(2R)-N-(4-chlorophenyl)-2-[cis-4-(6-fluoroquinolin-4-yl)cyclohexyl]propanamide | C24 H24 Cl F 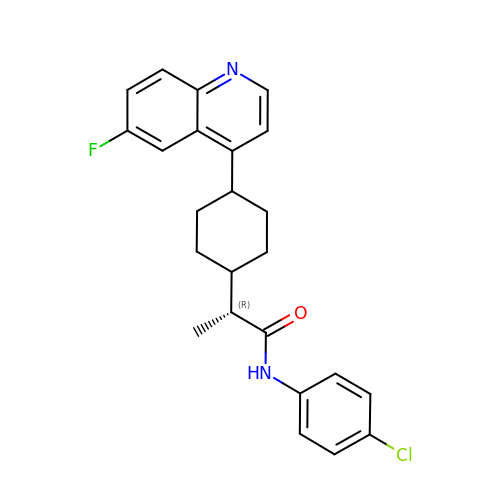N2 O | KRTIYQIPSAGSBP-ZACQAIPSSA-N> MFLLPYETTVCKTLYNPTGGGKLYPKQYVDQIENAIKKANVYLPIPPVDARNGETLEHSGQITPVDDFEDIKKFTQIVNIGDRDNPKLVVDARLYKKIEQRTGIPRIIQQNEWQFQYIRMALNIKLLREGPDFLHRLGDIPVKVFYNWISGILTQKYSLPPESTQAIWVICAVYYFAMQDDDLTEPGQERDRLIPIISRLTYIPAGFIADVIDTLGPLHNAGDLA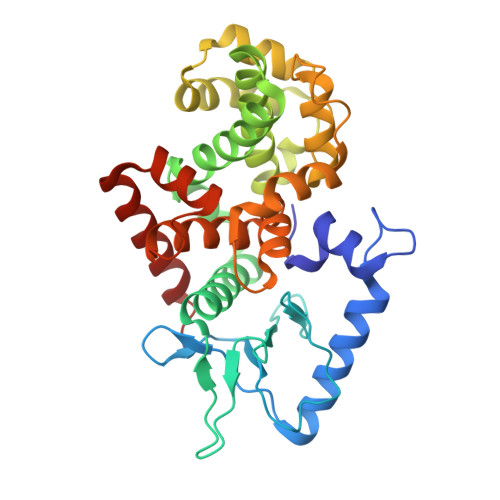YEISTNGRSIRMGKLKFSDLQLLVSPSWFGTASRENVGVALEHMPTYITLIYMALADRSYRKTVLSQKVEMISRSDDASRFINLVNEAVSSQFVK>MKYFLDSAILEEIRYAYENWAIDGVTTNPRHIMNSGKPFLTVLDEFASEFKGVENFPISVEINPHLDNAKDMVEEGTKIAKLSSNFVIKIPCTEPGLIAAKEFEKQGISTNVTLVFSPSQALQPARIGAKFVSPFVGWKENSGDDTTQYIQDIVNIYKNYNYNTEIIVAALRNGKQIVDAAKAGAHIVTCGFDVYKESFQHAFTDY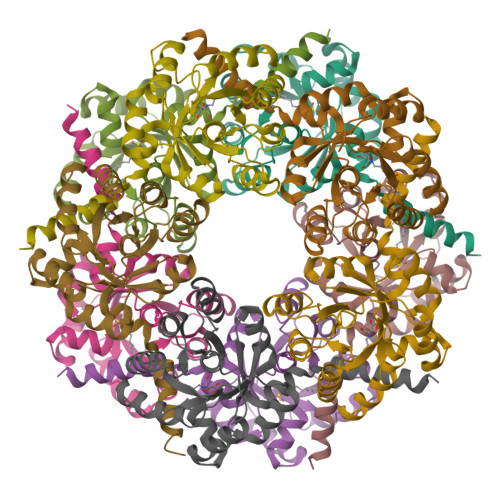GLNKFRNAWDNTV[10x]>[2x]MSAEVETSEGVDESEKKNSGALEKENQMRMADLSELLKEGTKEAHDRAENTQFVKDFLKGNIKKELFKLATTALYFTYSALEEEMERNKDHPAFAPLYFPMELHRKEALTKDMEYFFGENWEEQVQAPKAAQK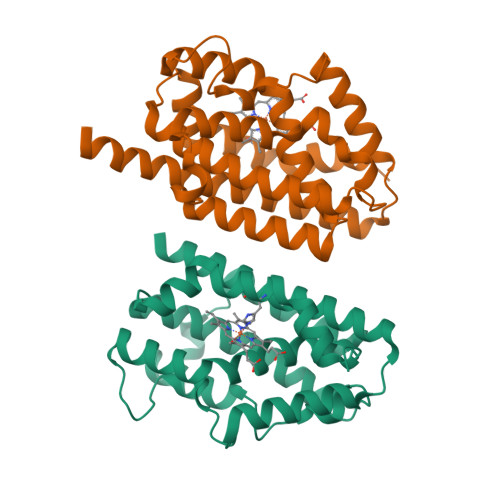YVERIHYIGQNEPELLVAHAYTRYMGDLSGGQVLKKVAQRALKLPSTGEGTQFYLFENVDNAQQFKQLYRARMNALDLNMKTKERIVEEANKAFEYNMQIFNELDQAGSTLARETLEDGFPVHDGKGDMRK>MAHHHHHHLVPRGSHETEQSVDLETVSVVGKSRPRATSGLLHTSTASDKIISGDTLRQKAVNLGDALDGVPGIHASQYGGGASAPVIRGQTGRRIKVLNHHGETGDMADFSPDHAIMVDTALSQQVEILRGPVTLLYSSGNVAGLVDVADGKIPEKMPENGVSGELGLRLSSGNLEKLTSGGINIGLGKNFVLHTEGLYRKSGDYAVPRYRNLKRLPDSHADSQTGSIGLSWVGEKGFIGVAYSDRRDQYGLPAHSHEYDDCHADIIWQKSLINKRYLQLYPHLLTEEDIDYDNPGLSCGFHDDDNAHAHTHSGRPWIDLRNKRYELRAEWKQPFPGFEALRVHLNRNDYRHDEKAGDAVENFFNNQTQNARIELRHQPIGRLKGSWGVQYLQQKSSALSAISEAVKQPMLLDNKVQHYSFFGVEQANWDNFTLEGGVRVEKQKASIQYDKALIDRENYYNHPLPDLGAHRQTARSFALSGNWYFTPQHKLSLTASHQERLPSTQELYAHGKHVATNTFEVGNKHLNKERSNNIELALGYEGDRWQYNLALYRNRFGNYIYAQTLNDGRGPKSIEDDSEMKLVRYNQSGADFYGAEGEIYFKPTPRYRIGVSGDYVRGRLKNLPSLPGREDAYGNRPFIAQDDQNAPRVPAARLGFHLKASLTDRIDANLDYYRVFAQNKLARYETRTPGHHMLNLGANYRRNTRYGEWNWYVKADNLLNQSVYAHSSFLSDTPQMGRSFTGGVNVKF[2x]

The zinc-uptake protein ZnuD is expressed under zinc-limiting conditions and was originally discovered in Neisseria meningitidis, where its expression is under the control of a zinc-sensing transcriptional factor, Zur14. ZnuD is an 82 kDa outer-membrane protein predicted to be a member of the TonB-dependent receptor (TbdR) family, requiring the mechanical energy derived from the TonB/ExbB/ExbD inner-membrane complex to couple nutrient uptake to the proton gradient across the inner-membrane. Characteristic of other TbdR family members, ZnuD consists of an amino-terminal plug domain (residues 1 to 147) obstructing the lumen of its own carboxy-terminal pore-forming domain (residues 148 to 734). Combined with molecular dynamic (MD) simulations, our structural findings suggest that ZnuD acquires free zinc ions using a series of binding sites that move zinc across the outer-membrane through a transient pore that requires TonB activation.

The high affinity of this TbdR for zinc is exemplified by the observation of a zinc ion bound to ZnuD despite no exogenous zinc addition during the purification. Indeed, all three ZnuD intermediate structures presented in this study contain a zinc ion buried in a high-affinity zinc-binding pocket. The metal ion captured within the high-affinity binding site is coordinated by four conserved residues (Asp-99, His-100, Glu-340 and His-499) located in a buried pocket that is sealed by the plug-apical loop and extracellular loop 6. The nature of the endogenous substrate bound to ZnuD in the crystal structures has been further characterized by X-ray absorption spectroscopy to confirm that the bound metal is a zinc ion. The absence of any metallophore within the binding site suggests that ZnuD is able to sequester and translocate free metal ions from the environment; however, it does not exclude any potential metallophore-binding activity as the neisserial TbdR FrpB/FetA has been reported to acquire its metal ligand either freely or presented through a siderophore. In addition, on binding its zinc ions on peripheral sites, the immunogenic loop 3 undergoes major conformational changes resulting in a switch between rigid (β-strand pairs) and flexible (α-helix) conformations. These two dynamic states of the external loop 3 illustrate how this loop adopts various conformations that would ultimately interfere with the surface/sequence availability of this epitope. Interestingly, the most immune-reactive epitopes reported to be targeted by the antibodies from convalescent patient overlaps with the extracellular loop 3, which camouflages the high-affinity zinc-binding pocket.>GSGMQPDMSLNVIKMKSSDFLESAELDSGGFGKVSLAFHRTQGLMIMKTVYKGPNCIEHNEALLEEAKMMNRLRHSRVVKLLGVIIE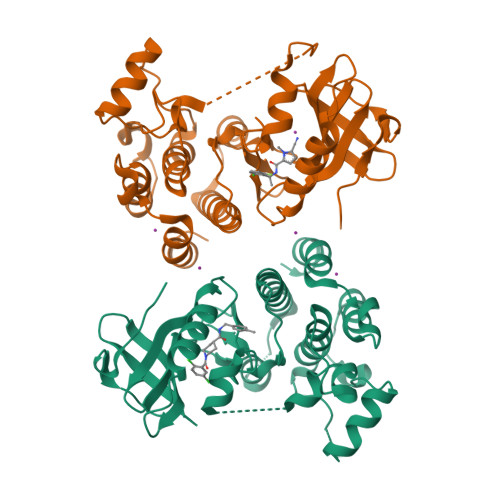EGKYSLVMEYMEKGNLMHVLKAEMSTPLSVKGRIILEIIEGMAYLHGKGVIHKDLKPENILVDNDFHIKIADLGLASFKMWSKLNNEEHNELREVDGTAKKNGGTLYYMAPEHLNDVNAKPTEKSDVYSFAVVLWAIFANKEPYENAIAEQQLIMAIKSGNRPDVDDITEYCPREIISLMKLCWEANPEARPTFPGIEEKFRPFYLSQLE[2x]>CLTSCPPLWTGFNGKCFRLFHNHLNFDNAENACRQFGLASCSGDELATGHLASIHSAESQAFLTELVKTSLPDLITGGWAPQVYIGMKVGSTNSDQTWTDGSSVDYDGWVSGEPNNGPNSRGAIAAGDYSRGFWADVYSNNNFKYICQLPCVHYT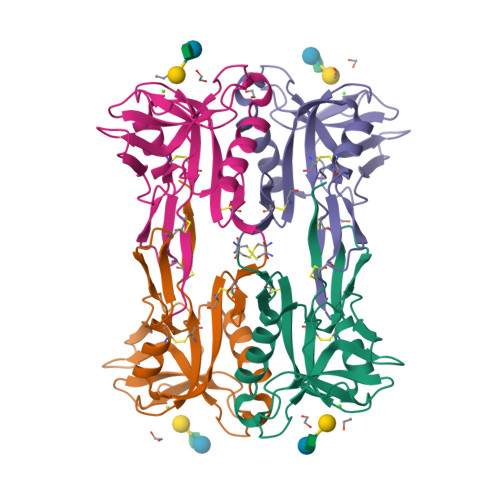LE[4x]>GSHMGGGGGIVLFVDFDYFYAQVEEVLNPSLKGKPVVVCVFSGRFEDSGAVATANYEARKFGVKAGIPIVEAKKILPNAVYLPMRKEVYQQVSSRIMNLLREYSEKIEIASIDEAYLDISDKVRDYREAYNLGLEIKNKILEKEKITVTVGISKNKVFAKIAADMAKPNGIKVIDDEEVKRLIRELDIADVPGIGNITAEKLKKLGINKLVDTLSIEFDKLKGMIGEAKAKYLISLARDEYNEPIRTRVRKSIGRIVTMK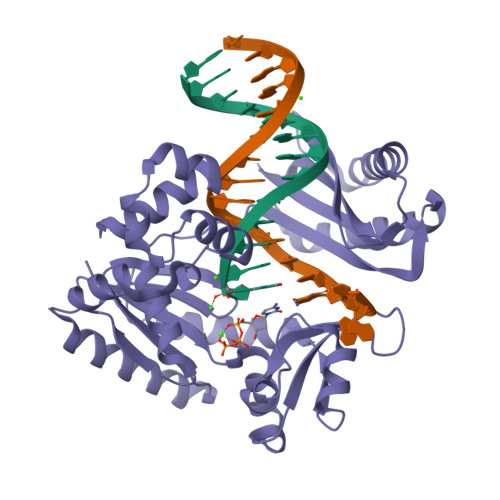RNSRNLEEIKPYLFRAIEESYYKLDKRIPKAIHVVAVTEDLDIVSRGRTFPHGISKETAYSESVKLLQKILEEDERKIRRIGVRFSKFIEAIGLDKFFDT[2x]ATAD2 is a non-canonical ATP-dependent histone chaperone and a major cancer target. From a structural standpoint, ATAD2 exhibits a conserved multidomain architecture comprising an N-terminal acidic domain, two AAA+ ATPase domains, a bromodomain, C-terminal domain, and an exceptionally long C-terminal linker (CTL) that bridges the bromo- and C-terminal domain. Unlike most other histone chaperones that do not require ATP for activity, ATAD2 stands out due to the presence of an ATP-dependent AAA+ ATPase domain. The AAA+ domain adopts a conserved structural fold found in the AAA+ ATPase superfamily, with each monomer consisting of a large α/β nucleotide binding domain (NBD) and a small α -helical bundle domain (HBD).

While processing of the ATAD2 structure yielded only a single major 3D class, the ATAD2-H3/H4 complex could be classified into three major 3D classes with resolutions of 3.8 Å (Class I), 4.3 Å (Class II), and 4.3 Å (Class III). Class III was similar to Class I but displayed an extra handle-like density that connected to one side of the AAA1 ring. This additional density was also observed as a weak signal in the 2D class averages. Although the identity of the extra density could not be definitively determined due to insufficient resolution, based on parallels to Abo1 and the general size and shape of the density, one possibility is that it corresponds to an ATAD2 bromodomain. A notable feature common to all classes of the ATAD2-H3/H4K5Q complex was the presence of an extra globular density that was unobserved in the ATAD2 alone structure. This density was situated on the top surface of the AAA+ ring close to the central pore and connected to a density resembling the substrate peptide observed in the ATAD2 structure. However, together with the XL-MS data that indicates crosslinking of the H3 tail to the ATAD2 AAA1 pore loops and the connectivity of the globular extra density to the H3 tail, we favor the idea that the structure represents a single H3/H4 dimer docked close to the AAA+ ring by the H3 tail. Superimposing the AAA+ domains from ATAD2 and ATAD2-histone complexes revealed that in the ATAD2-histone complexes, the P1 and P6 subunits moved away from each other, thus widening the seam cleft, and opening the AAA+ ring. The changes were most prominent in the asymmetric Class II conformation with less prominent changes in Class III and I. Consistent with potential movement of the N-terminal LD upon H3/H4 binding, examination of ATAD2 intramolecular crosslinks showed that the N-terminal LD crosslinked extensively with the nucleotide binding pocket, pore loop 1, bromodomain, and C-terminal linker (CTL) domain in the absence of histone H3/H4, but lost most of these crosslinks upon histone H3/H4 binding. Together, these data support the idea that H3/H4 binding to the bromo- and CTL domain might allosterically release the N-terminal LD from the P1/P6 seam, open up the AAA+ ring, and prime the AAA+ ring for activation.

>[6x]DRMKIGASLADVDPMQLDSSVRFDSVGGLSNHIAALKEMVVFPLLYPEVFEKFKIQPPRGCLFYGPPGTGKTLVARALANECSQGDKRVAFFMRKGADCLSKWVGESERQLRLLFDQAYQMRPSIIFFDQIDGLAPVRSSRQDQIHSSIVSTLLALMDGLDSRGEIVVIGATNRLDSIDPALRRPGRFDREFLFSLPDKEARKEILKIHTRDWNPKPLDTFLEELAENCVGYCGADIKSICAEAALCALRRRYPQIYTTSEKLQLDLSSINISAKDFEVAMQKMIPASQRAVTSPGQALSTVVKPLLQNTVDKILEALQRVFPHAEFRTNKTLDSDISCPLLESDLAYSDDDVPSVYENGLSQKSSHKAKDNFNFLHLNRNACYQPMSFRPRILIVGEPGFGQGSHLAPAVIHALEKFTVYTLDIPVLFGVSTTSPEETCAQVIREAKRTAPSIVYVPHIHVWWEIVGPTLKATFTTLLQNIPSFAPVLLLATSDKPHSALPEEVQELFIRDYGEIFNVQLPDKEERTKFFEDLILKQAAKPPISKKKAVLQALEVLPVAPPPEPRSLTAEEVKRLEEQEEYAPSYYHVMPKQNSTLVGDKRSDPEQNEKLKTPSTPVACSTPAQLKRKIRKKSNWYLGTIKKRRKISQAKDDSQNAIDHKIESDTEETQDTSVDHNETGNTGESSVEENEKQQNASESKLELRNNSNTCNIENELEDSRKTTACTELRDKIACNGDASSSQIIHISDENEGKEMCVLRMTQPTPSLVVDHERLKNLLKTVVKKSQNYNIFQLENLYAVISQCIYRHRKDHDKTSLIQKMEQEVENFSCSR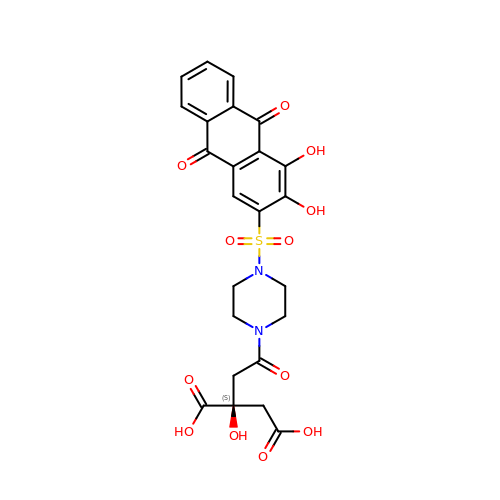(2~{S})-2-[2-[4-[3,4-bis(oxidanyl)-9,10-bis(oxidanylidene)anthracen-2-yl]sulfonylpiperazin-1-yl]-2-oxidanylidene-ethyl]-2-oxidanyl-butanedioic acid | C24 H22 N2 O12 S | PYHLNZSMOIJZLQ-DEOSSOPVSA-N>[2x]GLEFNSFQHQLRIQDQEFQEGFDGGWCLSVHQPWASLLVRGIKRVEGRSWYTPHRGRLWIAATAKKPS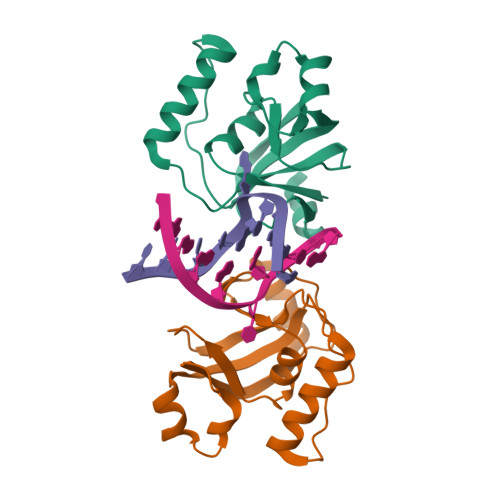PQEVSELQATYRLLRGKDVEFPNDYPSGCLLGCVDLIDCLSQKQFKEQFPDISQESDSPFVFICKNPQEMVVKFPIKGNPKIWKLDSKIHQGAKKGLMKQNKAV>[4x]GPMTSATSPIILKWDPKSLEIRTLTVERLLEPLVTQVTTLVNTSNKGPSGKKKGRSKKAHVLAASVEQATQNFLEKGEQIAKESQDLKEELVAAVEDVRKQGETMRIASSEFADDPCSSVKRGTMVRAARALLSAVTRLLILADMADVMRLLSHLKIVEEALEAVKNATNEQDLANRFKEFGKEMVKLNYVAARRQQELKDPHCRDEMAAARGALKKNATMLYTASQAF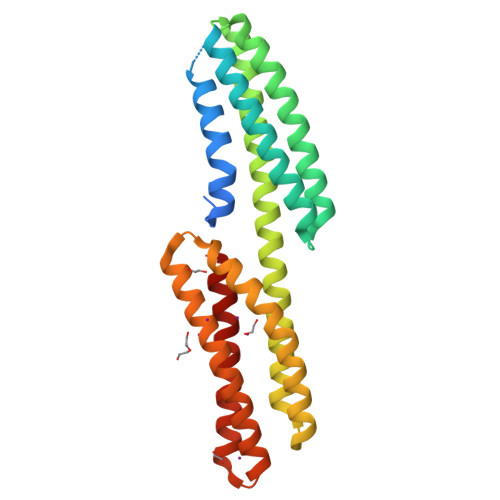LRHPDVAATRANRDYVFKQVQEAIAGISSAAQAT>[2x]MSKAFDLVVIGAGSGGLEAGWNAATLYGKRVAVVDVQTSHGPPFYAALGGTCVNVGCVPKKLMVTGAQYMDHLRESAGFGWEFDGSSVKANWKKLIAAKNEAVLDINKSYEGMFNDTEGLDFFLGWGSLE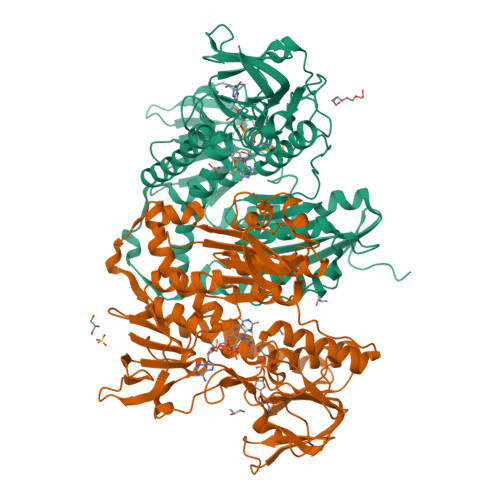SKNVVVVRETADPKSAVKERLQADHILLATGSWPQMPAIPGIEHCISSNEAFYLPEPPRRVLTVGGGFISVEFAGIFNAYKPPGGKVTLCYRNNLILRGFDETIREEVTKQLTANGIEIMTNENPAKVSLNTDGSKHVTFESGKTLDVDVVMMAIGRIPRTNDLQLGNVGVKLTPKGGVQVDEFSRTNVPNIYAIGDITDRLMLTPVAINEGAALVDTVFGNKPRKTDHTRVASAVFSIPPIGTCGLIEEVAAKEFEKVAVYMSSFTPLMHNISGSKYKKFVAKIVTNHSDGTVLGVHLLGDGAPEIIQAVGVCLRLNAKISDFYNTIGVHPTSAEELCSMRTPSYYYVKGEKMEKLPDSNL> KETAAAAFEAQHMDSSTSAASSSNYCNQMMKSRNLTKDRCKPVNTFVHESLADVQAVCSQKNVACANGQTNCYQSYSTMSITDCRETGSSKYPNCAYKTTQANKHIIVACEGNPYVPVHF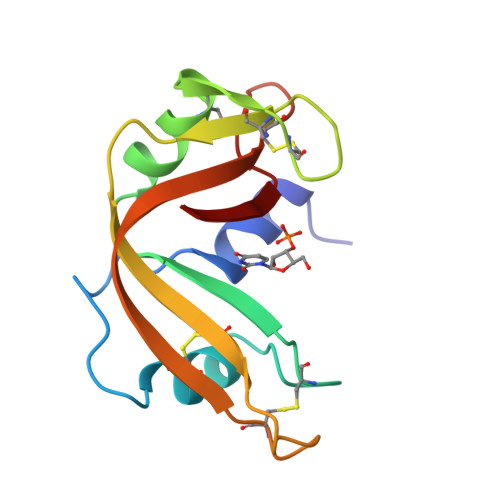DASV>NLLRRSGKRRRSESGSDSFSGSGGDSSASPQFLSGSVLSPPPGLGRCLKAAAAGECKPTVPDYERDKLLLANWGLPKAVLEKYHSFGVKKMFEWQAECLLLGQVLEGKNLVYSAPTSAGKTLVAELLILKRVLEMRKKALFILPFVSVAKEKKYYLQSLFQEVGIKVDGYMGSTSPSRHFSSLDIAVCTIERANGLINRLIEENKMDLLGMVVVDELHMLGDSHRGYLLELLLTKICYITRKSASCQADLASSLSNAVQIVGMSATLPNLELVASWLNAELYHTDFRPVPLLESVKVGNSIYDSSMKLVREFEPMLQVKGDEDHVVSLCYETICDNHSVLLFCPSKKWCEKLADIIAREFYNLHHQAEGLVKPSECPPVILEQKELLEVMDQLRRLPSGLDSVLQKTVPWGVAFHHAGLTFEERDIIEGAFRQGLIRVLAATSTLSSGVNLPARRVIIRTPIFGGRPLDILTYKQMVGRAGRKGVDTVGESILICKNSEKSKGIALLQGSLKPVRSCLQRREGEEVTGSMIRAILEIIVGGVASTSQDMHTYAACTFLAASMKEGK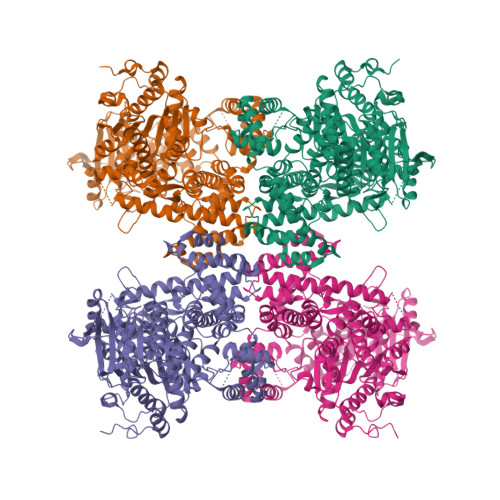QGIQRNQESVQLGAIEACVMWLLENEFIQSTEASDGTEGKVYHPTHLGSATLSSSLSPADTLDIFADLQRAMKGFVLENDLHILYLVTPMFEDWTTIDWYRFFCLWEKLPTSMKRVAELVGVEEGFLARCVKGKVVARTERQHRQMAIHKRFFTSLVLLDLISEVPLREINQKYGCNRGQIQSLQQSAAVYAGMITVFSNRLGWHNMELLLSQFQKRLTFGIQRELCDLVRVSLLNAQRARVLYASGFHTVADLARANIVEVEVILKNAVPFKSARKAVDEEEEAVEERRNMRTIWVTGRKGLTEREAAALIVEEARMILQQDLVEM[4x]>[2x]MRPPQFTRAQWFAIQAISLNPPRCTIAMRAINNYRWRCKNQNTFLRTTFANVVN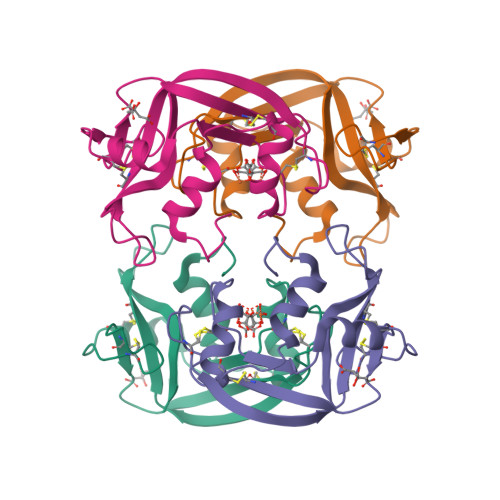VCGNQSIRCPHNRTLNNCHRSRFRVPLLHCDLINPGAQNISNCRYADRPGRRFYVVACDNRDPRDSPRYPVVPVHLDTTI>[2x]MFLAQEIIRKKRDGHALSDEEIRFFINGIRDNTISEGQIAALAMTIFFHDMTMPERVSLTMAMRDSGTVLDWKSLNLNGPIVDKHSTGGVGDVTSLMLGPMVAACGGYVPMISGRGLGHTGGTLDKLEAIPGFDIFPDDNRFREIIQDVGVAIIGQTSSLAPADKRFYATRDITATVDSIPLITGSILAKKLAEG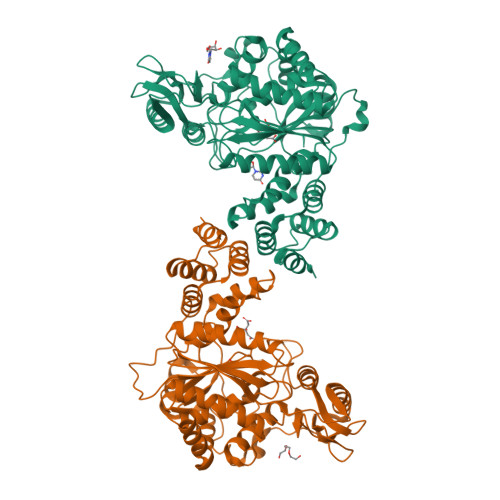LDALVMDVKVGSGAFMPTYELSEALAEAIVGVANGAGVRTTALLTDMNQVLASSAGNAVEVREAVQFLTGEYRNPRLFDVTMALCVEMLISGQLAKDDAEARAKLQAVLDNGKAAEVFGRMVAAQKGPSDFVENYDKYLPTAMLSKAVYADTEGFISAMDTRALGMAVVSMGGGRRQASDTIDYSVGFTDMARLGDSIDGQRPLAVIHAKDEASWQEAAKAVKAAIILDDKAPASTPSVYRRITE>[2x]EYNAPSEIKYIDVVNTYDLEEEASKVVPHGGFNYIAGASGDEWTKRANDRAWKHKLLYPRLAQDVEAPDTSTEILGHKIKAPFIMAPIAAHGLAHTTKEAGTARAVSEFGTIMSISAYSGATFEEISEGLNGGPRWFQIYMAKDDQQNRDILDEAKSDGATAIILTADSTNRDYPFGMPIVQRYLRGTAEGMYGASKQKISPRDIEEIAAHSGLPVFVKGIQHPEDADMAIKRGASGIWVSNHGARQLYE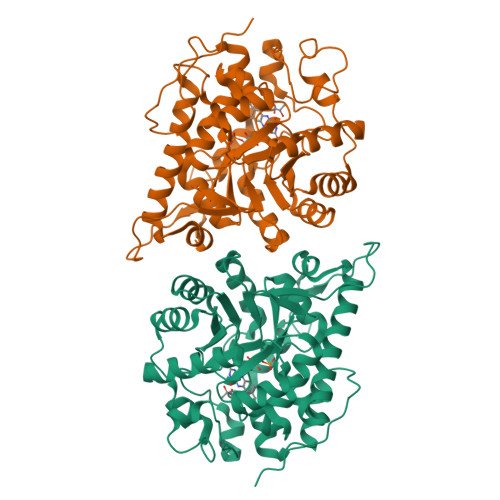APGSFDTLPAIAERVNKRVPIVFDSGVRRGEHVAKALASGADVVALGRPVLFGLALGGWQGAYSVLDYFQKDLTRVMQLTGSQNVEDLKGLDLFDNPYGYEYEYNAPSEIKYIDVVNTYDLEEEASKVVPHGGFNYIAGASGDEWTKRANDRAWKHKLLYPRLAQDVEAPDTSTEILGHKIKAPFIMAPIAAHGLAHTTKEAGTARAVSEFGTIMSISAYSGATFEEISEGLNGGPRWFQIYMAKDDQQNRDILDEAKSDGATAIILTADSTVSGNRDRDVKNKFVYPFGMPIVQRYLRGTAEGMSLNNIYGASKQKISPRDIEEIAAHSGLPVFVKGIQHPEDADMAIKRGASGIWVSNHGARQLYEAPGSFDTLPAIAERVNKRVPIVFDSGVRRGEHVAKALASGADVVALGRPVLFGLALGGWQGAYSVLDYFQKDLTRVMQLTGSQNVEDLKGLDLFDNPYGYEY> NW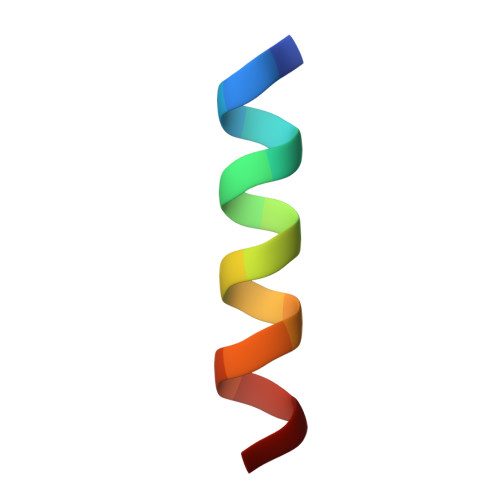KLLAKGLLIRERLKR>MAQVLRGTVTDFPGFDERADAETLRKAMKGLGTDEESILTLLTSRSNAQRQEISAAFKTLFGRDLLDDLKSELTGKFEKLIVALMKPSRLYDAYELKHALKGAGTNEKVLTEIIASRTPEELRAIKQVYEEEYGSSLEDDVVGDTSGYYQRMLVVLLQANRDPDAGIDEAQVEQDAQALFQAGELKWGTDEEKFITIFGTRSVSHLRKVFDKYMTISGFQIEETIDRETSGNLEQLLLAVVKSIRSIPAYLAETLYYAMKGAGTDDH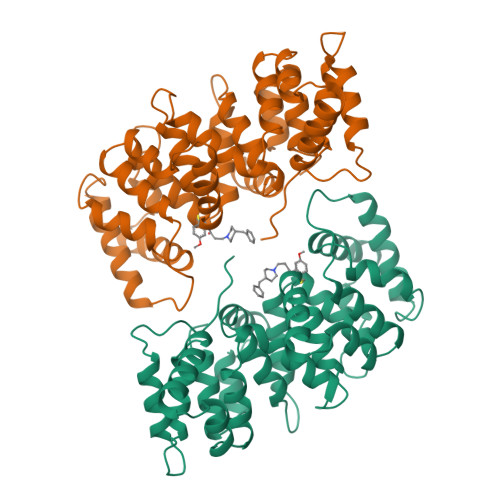TLIRVMVSRSEIDLFNIRKEFRKNFATSLYSMIKGDTSGDYKKALLLLCGEDD[2x]2,2-dimethylpropanenitrile | C5 H9 N | 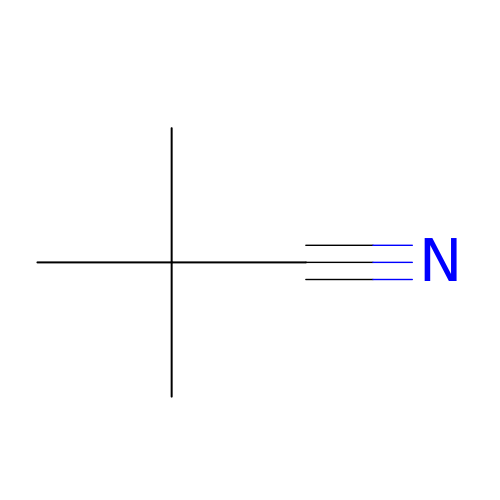JAMNHZBIQDNHMM-UHFFFAOYSA-N>[6x]MIIIGGSATNGIDESLSKILSIPLVKVENKIFPDGESYIRVPSSIRDEEVLLVQTTDYPQDKHLIELFLIAETIRDLGAKKLTAIVP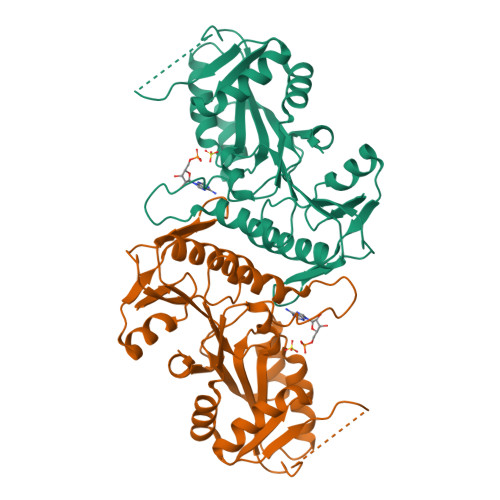YLAYSRQDRRFKDGEAISIKTILHILSEVGVNTLVVVEPHKPEELSYFKGELKIVHPYHQIARKIKEIIEDPFILAPDRGALDRARKIAEEINAPYSYIEKERDRTTGEVRIKEAPNINLKGKDVVIIDDIISTGGTIVQATRLAYSLGAKSVTAAAIHLLLVGGAKERLREVGVKTLIGTNTINVNDKDIITIDVSQSIALSL5-(4-{[1-(2-AMINO-5-FORMYL-7-METHYL-4-OXO-3,4,5,6,7,8-HEXAHYDROPTERIDIN-6-YL)ETHYL]AMINO}PHENYL)-5-DEOXY-1-O-{5-O-[(1,3-DICARBOXYPROPOXY)(HYDROXY)PHOSPHORYL]PENTOFURANOSYL}PENTITOL 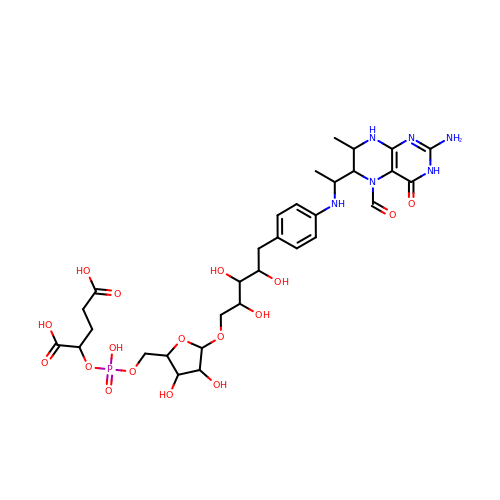| C31 H45 N6 O17 P | RMPHWTMYCVTPKB-BKULHTCLSA-N>[10x]MSLLSDLINLNLSDTTEKVIAEYIWIGGSGMDLRSKARTLPGPVSDPSKLPKWNYDGSSTGQAPGEDSEVIIYPQAIFRDPFRRGNNILVICDTYTPAGEPIPTNKRHDAAKVFSHPDVVAEETWYGIEQEYTLLQKDIQWPLGWPVGGFPGPQGPYYCGVGADKAFGRDIVDAHYKACLYAGINISGINGEVMPGQWEFQVGPSVGISAGDEVWAARYILERITEIAGVVVSFDPKPIQGDWNGAGAHTNYSTKSMRNDGGYEVIKTAIEKLGKRHKEHIAAYGEGNERRLTGRHETADINTFLWGVANRGASVRVGRDTEKAGKGYFEDRRPASNMDPYVVTSMIADTTILWKP

One such an example is glutamine synthetases (GSs) (EC 6.3.1.2), one of the most ancient functioning enzymes in existence and a central enzyme in nitrogen metabolism of all living organisms, catalyzing the formation of glutamine by condensation of glutamate with ammonia using ATP as an energy source. Decades of studies have established a striking notion that all three classes of GS enzymes, despite of dramatic differences in amino acid sequences and protein sizes, share quaternary geometry in dihedral symmetry assembled with two oligomeric rings. Considering that the active sites of GS are located at the clefts formed between two neighboring protomers within the same ring and distal to the ring-ring interface, each isolated GS subcomplex ring holds multiple integral catalytic sites. Cryo-EM structure determination of GS in both the catalytically active and inactive assembly states allows us to reveal an unanticipated self-assembly-induced disorder-order transition paradigm, in which the remote interactions between two subcomplex entities significantly rigidify the otherwise structurally fluctuating active sites, thereby regulating activity.

MALS analysis shows the GSII from Glycine max being largely a homogeneous decamer in solution. When supplied with ammonium chloride, the stable decamer-adopting GmGSβ2 demonstrated significant GS activities. To elucidate the detailed mechanism of how the interactions between two GSII pentameric rings remotely trigger enzymatic activity, we next employed single-particle cryo-EM imaging technique and first determined the structures of GmGSβ2 decamer, as well as that of the CsGSIb that adopts decameric configuration (thereafter named as CsGSIbDec). 3D classifications of 104,717 and 43,876 particles for GmGSβ2 and CsGSIbDec, respectively, revealed that both molecules were arranged in D5 symmetry with two pentameric rings stacked in a head-to-head manner, a strikingly conserved structural feature for type II GS species. Refinement of the GmGSβ2 and CsGSIbDec structures yielded maps with an average resolution of 2.9 Å and 3.3 Å, respectively (Figure 3—figure supplements 1–3), with literally identical dimensions of 115 Å x 115 Å x 95 Å. The active sites of GmGSβ2, CsGSIbDec are structurally highly similar to each other, as well as to that of the maize GSII, suggesting the catalysis mechanisms of these plant GSIIs are essentially identical. The overall buried inter-ring surfaces for both GmGSβ2 and CsGSIbDec amount to ~2000 Å2, that is approximately only 400 Å2 per individual monomer–monomer interaction. This highlights the weakness of the inter-ring contacts, characteristic of type II GS.> DRHHHHHHKLAPVQSQGSQNKLLLVSFDGFRWNYDQDVDTPNLDAMARDGVKARYMTPAFVTMTSPCHFTLVTGKYIENHGVVHNMYYNTTSKVKLPYHATLGIQRWWDNGSVPIWITAQRQGLRAGSFFYPGGNVTYQGVAVTRSRKEGIAHNYKNETEWRANIDTVMAWFTEEDL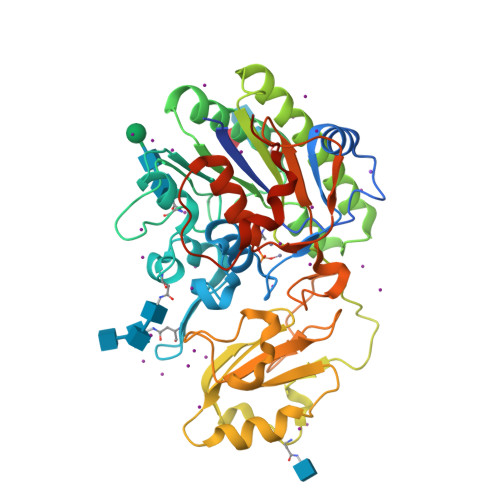DLVTLYFGEPDSTGHRYGPESPERREMVRQVDRTVGYLRESIARNHLTDRLNLIITSDHGMTTVDKRAGDLVEFHKFPNFTFRDIEFELLDYGPNGMLLPKEGRLEKVYDALKDAHPKLHVYKKEAFPEAFHYANNPRVTPLLMYSDLGYVIHGRINVQFNNGEHGFDNKDMDMKTIFRAVGPSFRAGLEVEPFESVHVYELMCRLLGIVPEANDGHLATLLPMLHTESALPPDGRPTLLPKGRS5'-(4-cyclopropyl-6-methoxypyrimidin-5-yl)-N-{[4-(ethylsulfonyl)phenyl]methyl}spiro[cyclopentane-1,3'-pyrrolo[3,2-b]pyridine]-1'(2'H)-carboxamide 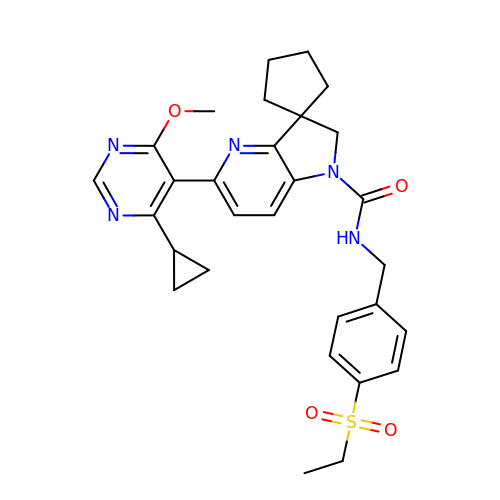| C29 H33 N5 O4 S | PWIXSNKHPMGRRW-UHFFFAOYSA-N>[2x]AAKEVCYGQ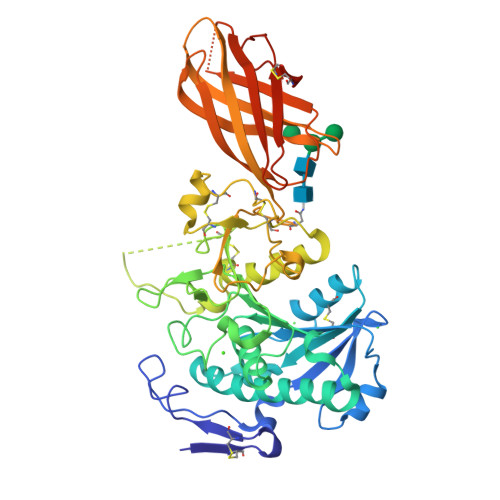LGCFSDEKPWAGTLQRPVKLLPWSPEDIDTRFLLYTNENPNNFQLITGTEPDTIEASNFQLDRKTRFIIHGFLDKAEDSWPSDMCKKMFEVEKVNCICVDWRHGSRAMYTQAVQNIRVVGAETAFLIQALSTQLGYSLEDVHVIGHSLGAHTAAEAGRRLGGRVGRITGLDPAGPCFQDEPEEVRLDPSDAVFVDVIHTDSSPIVPSLGFGMSQKVGHLDFFPNGGKEMPGCKKNVLSTITDIDGIWEGIGGFVSCNHLRSFEYYSSSVLNPDGFLGYPCASYDEFQESKCFPCPAEGCPKMGHYADQFKGKTSAVEQTFFLNTGESGNFTSWRYKVSVTLSGKEKVNGYIRIALYGSNENSKQYEIFKGSLKPDASHTCAIDVDFNVGKIQKVKFLWNKRGINLSEPKLGASQITVQSGEDGTEYNFCSSDTVEENVLQSLYPCEFVEHHHHHHHH(2R,3R,4R,5S)-2-(hydroxymethyl)-1-{9-[4-(methoxymethyl)-1H-1,2,3-triazol-1-yl]nonyl}piperidine-3,4,5-triol 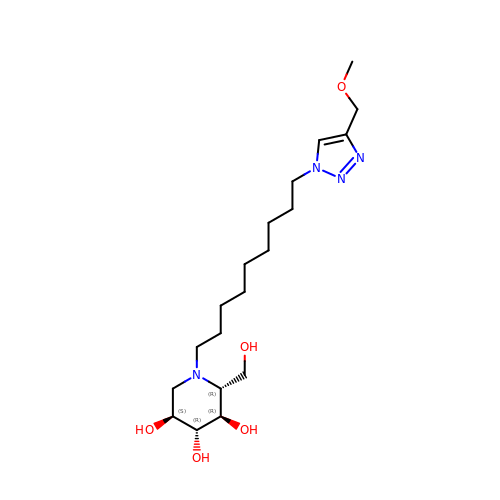| C19 H36 N4 O5 | XGVWMUFCIMYWGD-FCGDIQPGSA-N>MASVVAIHEAETADYILDVLVEGVKAKAGDTVEIPLKFENVPSHGIQSFNLSLYYDSKAIEVLKVEPGSIITDPANNFDYNIVYKDSEIVFLFDDDKQKGEGLIKTDGVFAKLTVRIKPDIFKDSGSTKKYSLITFGESNFCDFDLKPILAVLKEGKVEIEKLEHHHHHH[2x];>MWNKAVIGDVNADGVVNISDYVLMKRYILRIIADFPADDDMWVG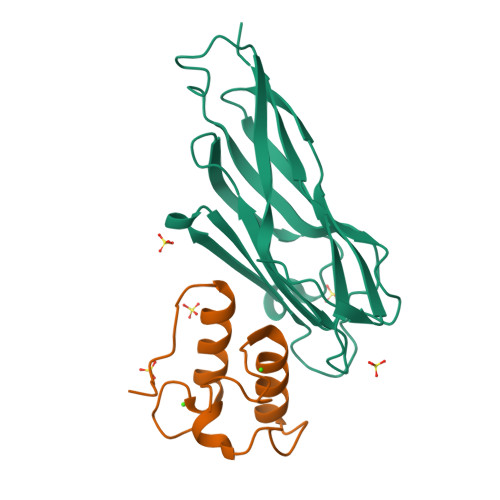DVNGDNVINDIDCNYLKRYLLHMIREFPKNSYNSAPTF[2x]The centrosome, which plays a central role as the main microtubule (MT)-organizing center for animal cell division, is a membraneless organelle composed of a pair of orthogonally arranged MT-derived apparatus, called centrioles, and the surrounding pericentriolar material (PCM). Here, we demonstrate that two of the human PCM scaffolds, Cep63 and Cep15212–14, cooperate to generate a higher-order cylindrical self-assembly capable of recruiting their downstream components, such as Plk4, a key regulator of centriole duplication. Here we showed that two centrosomal scaffolds, Cep63 and Cep152, cooperatively interact with each other to generate a heterotetrameric α-helical bundle, which in turn self-assembles into a higher-order cylindrical architecture that resembles the localization morphology of endogenous Cep152 detected around a centriole. Remarkably, short (~50 residues) coiled-coil heterotetramerization regions of Cep63 and Cep152 and their neighboring hydrophobic motifs (i.e., Cep63 P1 and Cep152 M4d) were necessary and sufficient to generate the cylindrical self-assembly capable of recruiting its guest molecules critical for centriole duplication in vivo.

As expected, a smaller Cep63 P1b5(502–541)•Cep152 M4e15(1205–1257) complex lacking the hydrophobic motifs maintained its 2:2 heterotetrameric state (expected MW 25.56 kDa) without forming any detectable high MW complex. In particular, identical hydrophobic residues in the parallelly aligned Cep152 helices appeared to constitute the backbone of the bundle by engaging in pairwise ladder-like interactions (top). Cep63 helices did not directly interact with each other, but rather interacted with both Cep152 helices in an antiparallel fashion (middle and bottom). Since Cep63 P1 and Cep152 M4d form an elongated four-helix bundle that may serve as a building block for the self-assembly, the mode of interaction between the bundles may likely determine the directionality of the assembly that positions Cep152 at the outskirts of the Cep63 arrangement.

>AHMTRFLEEEELRSHHILERLDAHIEELKRESEKTVRQFTALKGGGSEGALEELRGQYIKAVKKIKCDMLRYIQESKERAAEMVKAEVLRERQE[4x]> YPKGV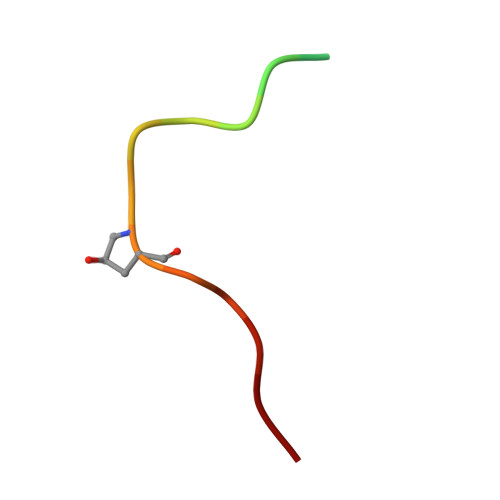PIPPSAPSKRHN>SMSATRRVHIYPFEGEVDGLEIHPKFAELRETDPLARVRLPYGGEGWMVTRYDDVRAANSDPRFSRAQIGEDTPRTTPLARRSDTILSLDPPEHTRLRRLLSKAFTARRMGAMQSWLEELFAGLLDGVERTGHPADIVRDLAQPFTIAVICRLLGVPYEDRGRFQHWSEVIMSTTAYSKEEAVSADASIRAYLADLVSARRAAPHDDLLGVLVSARDDDDRLTEDELITFGVTLLVAGHETSAHQLGNMVYALLTHEDQLSLLREQPELLPRAVEELLRFVPLGNGVGNARIALEDVELSGGTVRAGEGVVAAAVNANRDPRAFDDPDRLDITREKNPHLAFGHGAHYCLGAQLARMELRVAIGGLLE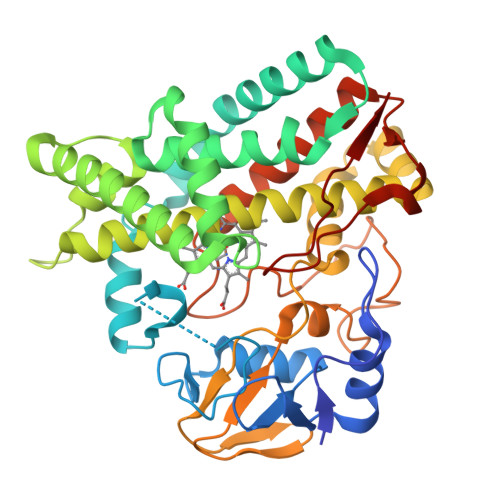RFPGLRLAVPADQVEWKTGGLFRGPQRLPIAW[2x]> GSMAWKIRFYSGLNQGAEVSLGEGRVALGSDPLQADLVLLDEGIAAVHLVLEVDAQGVRLLEWAEGCEPRQDGQAQVAGAILQALAGQTCGPLRWTFCDPQRSFPERFPEAEVQTAPVRRK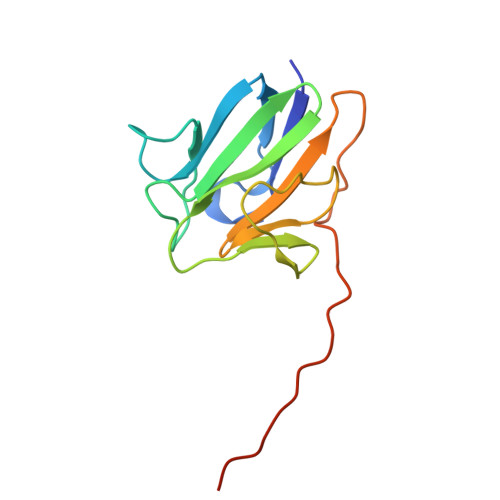SSARAGG> GHMTQAVEAGEKTVEQFVQALNKGDYNKAAEMTSKKAANKSALSEKEILDKYQNIYGAADVKGLQISNLKVDKKDDSTYSFSYKAKMNTSLGELKDLSYKGTLDRNDGQTTINWQPNLVFPEMEGNDKVSLTTQEAARGNIIDRNGEPLATTGKLKQLGVVPSKLGDGGEKTANIKAIASSFDLTEDAINQAISQSWVQPDYFVPLKIIDGATPELPAGATIQEVDGRYYPLGEAAAQLIGYVGDITAEDIDKNPELSSNGKIGRSGLEMAFDKDLRGTTGGKLSITDADGVEKKVLIEHEVQNGKDIKLTIDAKAQKTAFDSLGGKAGSTVATTPKTGDLLALASSPSYDPNKMTNGISQEDYKAYEENPEQPFISRFATGYAPGSTFKMITAAIGLDNGTIDPNEVLTINGLKWQKDSSWGSYQVTRVSDVSQVDLKTALIYSDNIYTAQETLKMGEKKFRTGLDKFIFGEDLDLPISMNPAQISNEDSFNSDILLADTGYGQGELLINPIQQAAMYSVFANNGTLVYPKLIADKETKDKKNVIGETAVQTIVPDLREVVQDVNGTAHSLSALG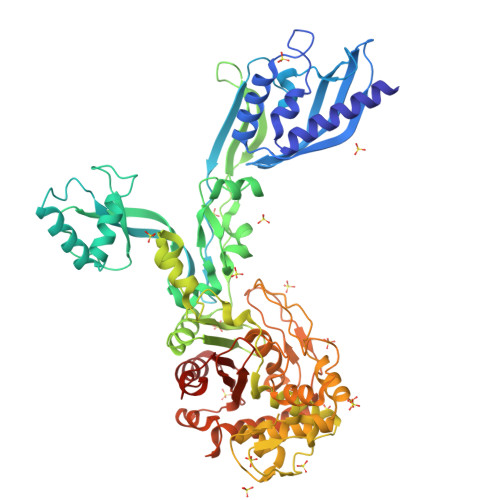IPLAAKTGTAEIKEKQDVKGKENSFLFAFNPDNQGYMMVSMLENKEDDDSATKRASELLQYLNQNYQ> LTPEVGELIEKVRKAHQETFPALCQLGKYTTNNSSEQ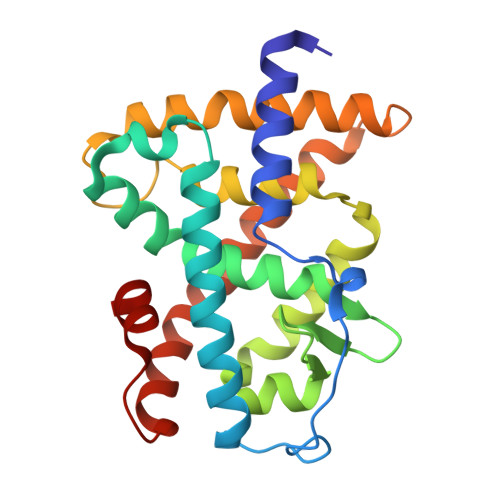RVSLDIDLWDKFSELSTKCIIKTVEFAKQLPGFTTLTIADQITLLKAACLDILILRICTRYTPEQDTMTFSDGLTLNRTQMHNAGFGPLTDLVFAFANQLLPLEMDDAETGLLSAICLICGDRQDLEQPDRVDMLQEPLLEALKVYVRKRRPSRPHMFPKMLMKITDLRSISAKGAERVITLKMEIPGSMPPLIQEMLE> GMAFMEKIFPDILEAIRNEEIIKESKKIPMPYFGLFALVIFDKVKELGSETSLYEIGEEFGKMLSPKNIEELKKIFKLMNFGDLEIDENKILLKNPPYKIKLSNPPYQWVSKEEPIHDFIAGILAGCLEEIFYYYFVVNEVEC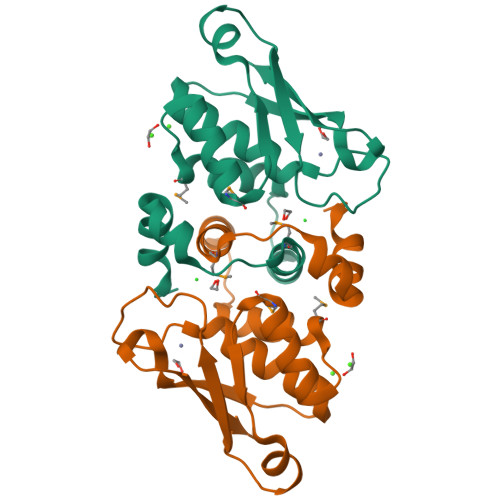VSQGKDKCVFEVKEVDELNK>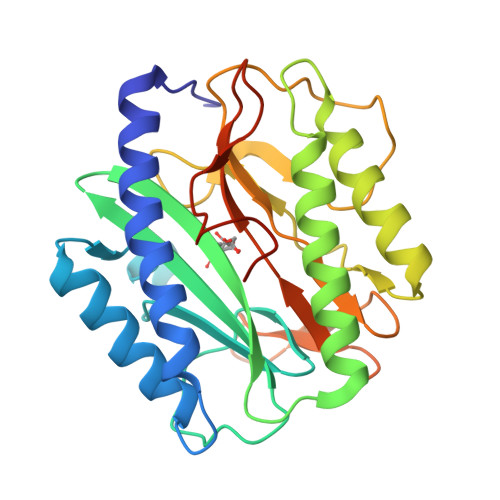[3x]MITLKSPREIEMMDESGELLADVHRHLRTFIKPGITSWDIEVFVRDFIESHGGVAAQIGYEGYKYATCCSINDEICHGFPRKKVLKDGDLIKVDMCVDLKGAISDSCWSYVVGESTPEIDRLMEVTKKALYLGIEQAQVGNRIGDIGHAIQTYVEGEGYGVVRDFVGHGIGPTIHESPMIPHYGEAGKGLRLKEGMVITIEPMVNTGTWRMKMDPNGWTAYTEDGGLSCQYEHSLAITKEGPRILTSQGEELTYLEHHHPPTEE> SMASQGGDSGNSKQESNSKDKEVKKIGITQLVEHPALDATRTGFVKALEKNGFKDGENIDIDFQNAQNDMPTTQSIASKFASDKKDLIFAISTPSAQAAFNATKDIPILITAVSDPVAAGLVKTLEKPGTNVSGTSDFVSVDKGLELLKIFAPKAKTIGVMYNTSEVNSKVQVDALKEYASKNGFKVVEKGITTSNEVNQGISSLVGKIDVLYVPTDNLVASSMPIVSKIATENKIPVIAAESGPVEKGALACQGINYEKLGYKTGEMAVKILNGESVSDMPVATSDDTDIIVNEDILKALGMEKPSNENISYVKTKQE

The C. difficile antigen CD0873 is annotated as a substrate-binding protein component (SBP) of an ATP-binding cassette (ABC) transporter and is an immunoreactive protein in human infection. We have previously shown, using both genetic and cellular approaches, that CD0873 is a surface-exposed lipoprotein and an adhesin of C. difficile. CD0873 assumes a typical Class I or Cluster B SBP-fold. The protein possesses two domains, each consisting of an α-β-α sandwich joined by three loops that form a hinge.

The closed, ligand-bound structure was determined to a resolution of 1.35 Å; the semi-open, ligand-bound structure was determined to 1.80 Å; and the open, ligand-free structure was determined to 2.50 Å. The closed structure has a tyrosine molecule (retained during purification) bound. The structural and biochemical information reported in this study demonstrates that tyrosine is the ligand of CD0873. The exquisite specificity of CD0873 for tyrosine is likely achieved through the tyrosine OH group. This is hydrogen bonded to the side chain of Glu-263, and to the main chain carbonyls of Val-235 and Pro-236 through a water molecule. In VC_1101 and SP1069, Glu-263 is replaced by an alanine: the lack of an appropriate hydrogen bond donor in these proteins explains their preference for more hydrophobic amino acids. Gln-284 in SP1069 aids binding of tryptophan through a hydrogen bond to the indole nitrogen; this glutamine is replaced by a tyrosine in CD0873 and VC_1101, which prevents binding of the larger tryptophan side chain through steric hindrance. CD0873 has a tyrosine molecule bound, whereas VC_1101 has phenylalanine bound and SP1069 has tryptophan bound. Comparison of the structures shows that the proteins share a common mechanism of binding to the amino and acid groups, but show sequence differences that account for their side chain preferences. DSF analysis strongly suggested, in agreement with the crystallization studies, that CD0873 specifically binds tyrosine (p < 0.0001).> RHKKL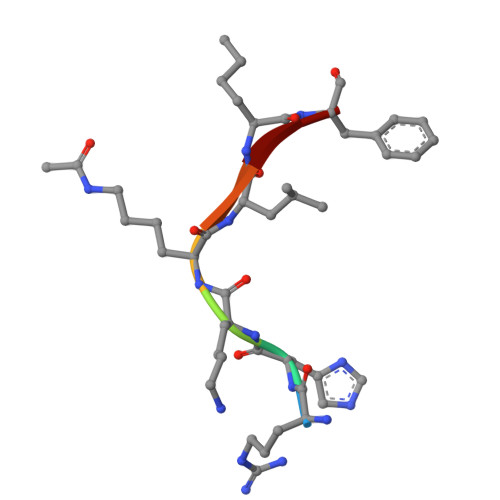LF>[48x]MSCECSGSALTCCPDKNYVQDKVCSPWSGTVVATAITNVLYNNNINQNMIGTGFVRYDVGPAPITLTVLDAAGATIDTQTLN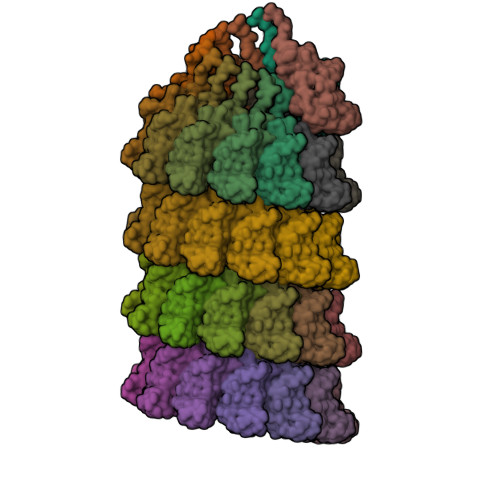PGTSIAFTYRRFVTIEVTLPAATAGTYQGEFCITTRYPLS> MSVSEIFVELQGFLAAEQDIREEIRKVVQSLEQTAREILTLLQGVHQGAGFQDIPKRCLKAREHFGTVKTHLTSLKTKFPAEQYYR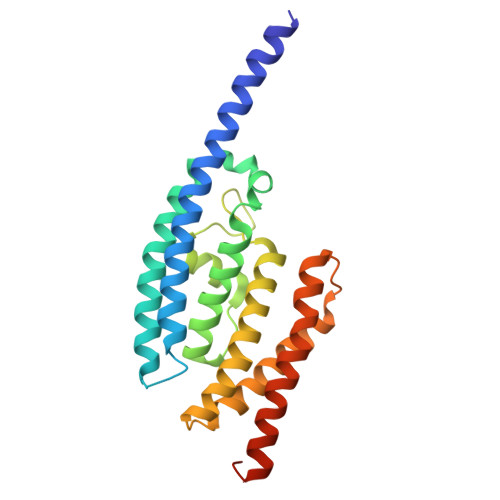FHEHWRFVLQRLVFLAAFVVYLETETLVTREAVTEILGIEPDREKGFHLDVEDYLSGVLILASELSRLSVNSVTAGDYSRPLHISTFINELDSGFRLLNLKNDSLRKRYDGLKYDVKKVEEVVYDLSIRGFNKETAAACVEK>GPLGSEEDVPENNGILISIKEVINAEFSRDGTIHSSELKGVLELRINDHDLSHSNLKLADSIDVRDKSFQFKTHPNIDKQSFLSTKLISLRDKSKAFPANDQSLGVLRWRKVAPAEDDSLIPLTLTTWVSPSESQQGFDVIIEYESVLETELADVIFTIPVFPQEPVDINTESSTCSDAEVVNMDQEMGTSIKISKIAANDAGALAFTIEAPYEDALYPMTVSFQESTRDKLAKSFTGMAIQSVVMANDHDQELPY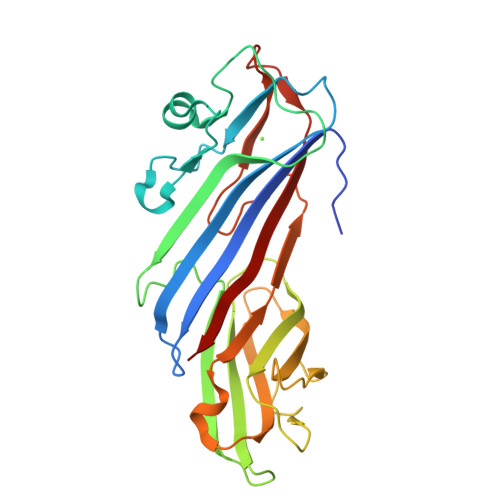DVITSLKSDEYLVQ[8x]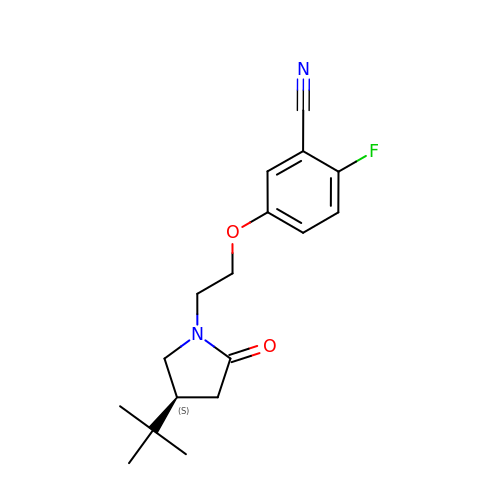5-[2-[(4~{S})-4-~{tert}-butyl-2-oxidanylidene-pyrrolidin-1-yl]ethoxy]-2-fluoranyl-benzenecarbonitrile | C17 H21 F N2 O2 | ZXBQUZQFTWNQON-CYBMUJFWSA-N>MAHHHHHHMSKLAGKVAIVTGASKGIGAAIAKALADEGAAVVVNYASSKAGADAVVSAITEAGGRAVAVGGDVSKAADAQRIVDTAIETYGRLDVLVNNSGVYEFAPIEAITEEHYRRQFDTNVFGVLLTTQAAVKHLGEGASIINISSVVTSITPPASAVYSGTKGAVDAITGVLALELGPRKIRVNAINPGMIVTEGTHSAGIIGSDLEAQVLGQTPLGRLGEPNDIASVAVFLASDDARWMTGE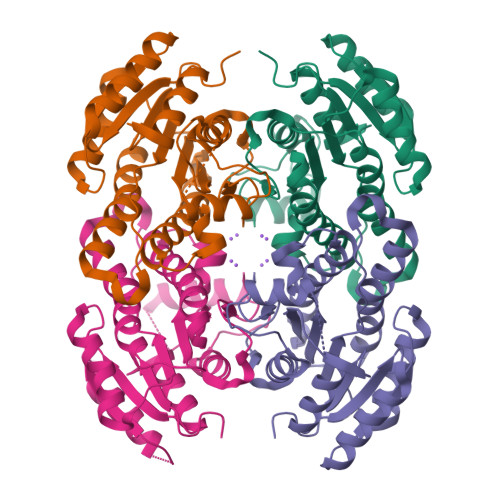HLVVSGGLN[4x]> GSTYVQALFDFDPQEDGELGFRRG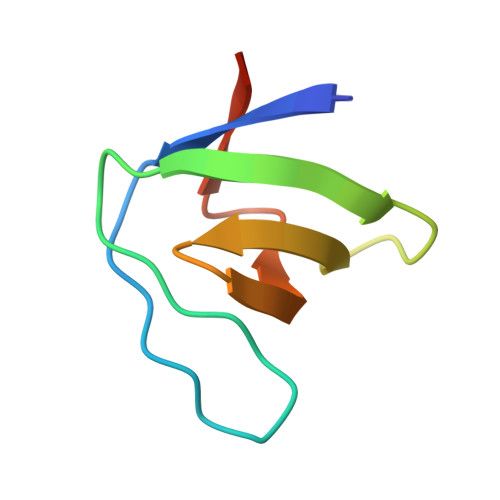DFIHVMDNSDPNWWKGACHGQTGMFPRNYVTPVNRNV>[28x]MAHHHHHHMSYKSHQLIKDHDVKWVDLRFTDTKGKQQHVTMPARDALDDEFFEAGKMFDGSSIAGWKGIEASDMILMPDDSTAVLDPFTEEPTLILVCDIIEPSTMQGYERDPRNIAKRAEEYLKSTGIGDTVFVGPEPEFFIFDEVKFKSDISGSMFK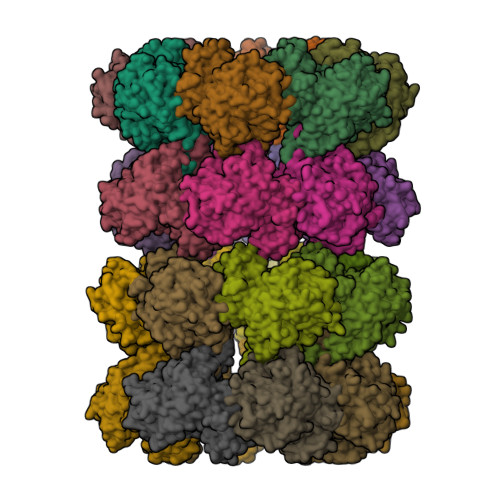IFSEQASWNTDADIESGNKGHRPGVKGGYFPVPPVDHDHEIRTAMCNALEEMGLVVEVHHHEVATAGQNEIGVKFNTLVAKADEVQTLKYCVHNVADAYGKTVTFMPKPLYGDNGSGMHVHMSISKDGKNTFAGEGYAGLSETALYFIGGIIKHGKALNGFTNPSTNSYKRLVPGFEAPVMLAYSARNRSASIRIPYVSSPKARRIEARFPDPAANPYLAFAALLMAGLDGIQNKIHPGDAADKNLYDLPPEEAKEIPQVCGSLKEALEELDKGRAFLTKGGVFTDEFIDAYIELKSEEEIKVRTFVHPLEYDLYYSV>[4x]MKKKGSVVIVGRINLSGDTAYAQQTRGEEGCQETSQTGRDKNQVEGEVQIVSTATQTFLATSINGVLWTVYHGAGTRTIASPKGPVTQMYTNVDKDLVGWQAPQGSRSLTPCTCGSSD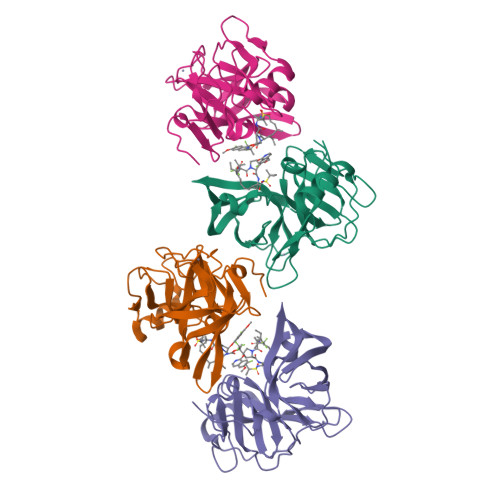LYLVTRHADVIPVRRRGDSRGSLLSPRPISYLKGSSGGPLLCPAGHAVGIFRAAVCTRGVAKAVDFIPVESLETTMRSPAIRAPSTSLRPHSSTTTTTTEI>GSHMPRDYTPICDNIVKLTLTSDGKSITLYGLQYGNYIITNRHLFRLNNGTLTIESKNGTYTIADSKTLEVHLIEGKDLVILKMPDSVPAADTTLKFKKPVENEEVVLVSRDFSTPEPKCLVSESSKITPDNDGTFWKHSIPTKDGEA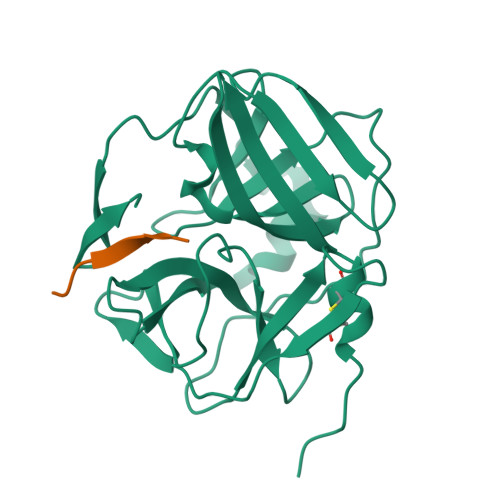GLPLVSTKDGTVVGLHSASNFNNTNFYFTAIPENFMELLNDESKRKWIKGWHLTSNSVEWGGHKVFMDK[4x];>TENLYFQGT[4x]DMT1 is a member of the conserved SLC11/NRAMP family, which is expressed in all kingdoms of life and which constitutes transporters for transition metals such as Fe2+ and Mn2+. SLC11 transporters are monomers and their fold resembles the general organization of a branch of the APC (amino acid-polyamine-cation) superfamily containing transporters for amino acids and glucose. The substrate binding site is located in the center of the protein formed by residues in unwound regions of the pseudo-symmetry related α-helices 1 and 6. In metal ion transporters of the SLC11 family the binding-site contains side-chains of conserved aspartate and asparagine residues located on α1 which are directly involved in ion interactions and a methionine residue on α6, which acts as soft ligand that is capable of coordinating transition metal ions but not Ca2+.

For that purpose, we have soaked crystals of EcoDMT with Br-BIT and oBr-BIT and collected multiple datasets at a wavelength corresponding to the anomalous absorption edge of bromine. Whereas we were unable to detect bromine in the anomalous maps of oBr-BIT containing crystals, the majority of datasets collected from crystals soaked with Br-BIT displayed a single strong peak in the anomalous difference density at equivalent positions, which aided the localization of the bound inhibitor. In this structure, EcoDMT adopts the same substrate-free outward-facing conformation that has previously been observed in datasets of the protein in absence of the inhibitor. In this conformation, a funnel-shaped aqueous pocket of the protein leads from the extracellular solution to the substrate binding site. The inhibitor is bound at the base of this pocket as defined by the anomalous difference density that constrains the position of the covalently bound Br-atom and by residual density in the 2Fo-Fc omit map that was calculated with phases from a model not containing the inhibitor. The omit map of the EcoDMT Br-BIT complex displays density for the aromatic ring and for the isothiourea group located close to the metal ion binding site (termed proximal isothiourea group), whereas the other group (the distal isothiourea group) is not defined in the electron density reflecting its increased conformational flexibility. The aromatic group is stacked between α-helices 6 and 10 contacted by the side chains of residues Ala 231, Leu 410, Ala 409 and Leu 414. The proximal isothiourea group is located in a narrow pocket in interaction distance to the conserved Asp 51 and Asn 54 in the unwound part of α−1 and to Gln 407 on α−10, which were shown to contribute to the coordination of transported metal ions. The distal isothiourea group is located in the wider entrance of the cavity and might thus adopt different conformations, which is consistent with its undefined position in the electron density.

> DLSLSDINSTVEVPEGHSFWKTLLAYSGPGALVAVGYMDPGNWSTSITGGQNFQYLLLSIIVISSLLAMLLQNMAAKLGIVCQLDLAQAIRARTSRRLGFIFWILTELAIMATDIAEVIGAAIALYLLFKIPIFLAVVITVLDVFLLLLLNRIGFRKIEALVVCLIFVILFVFLYQIILSQPAWHQVAKGLIPSWASVQTSPKIGGQTPLSASLGIIGATIMPHNLFLHSAISQSRKIDRTDSSKVAEAVRFSNWDSNIQLSLAMVVNALLLIMGVAVFKSGAVQDPSFFGLYQALSNPDMVSNPVLAEAARSGVLSTLFAVALLASGQNSTITGTITGQVIMEGFIHLRLPLWLRRLVTRLIAIIPVVVCVAITSHQGSLDEHQALNNLMNNSQVFLALALPFSIVPLLMLTDSAAQMGNQFKNTRWVKVMGWLTVIILTLLNLISISSQIAGFFGDNPSSQDLLLSQVISIGIILAMIGLLIWTIIDIRRFT>QEGDFPMPFISAKSSPVIPLDGSVKIQCQAIREAYLTQLMIIKNSTYREIGRRLKFWNETDPEFVIDHMDANKAGRYQCQYRIGHYRFRYSDTLELVVTGLYGKPFLSADRGLVLMPGENISLTCSSAHIPFDRFSLAKEGELSLPQHQSGEHPANFSLGPVDLNVSGIYRCYGWYNRSPYLWSFPSNALELVVTAIDG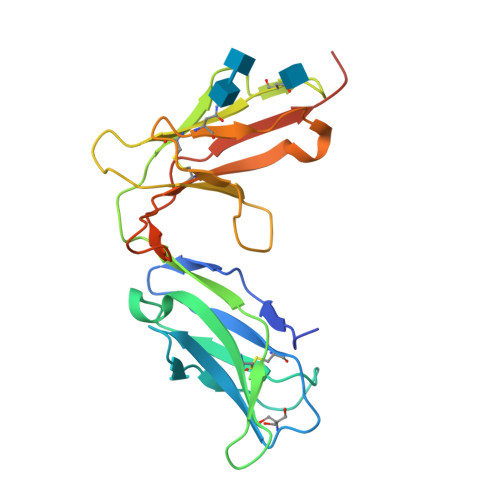RAHHHHHH[2x]> RVPPPPPCCHPRLSLHRPALEDLLLGSEANLTCTLTGLRDASGATFTWTPSSGKSAVQGPPERDLCGCYSVSSVLPGSAQPWNHGETFTCTAAHPELKTPLTATLSKSGNTFRPEVHLLPPPSEELALNELVTLTCLARGFSPKDVLVRWLQGSQELPREKYLTWASRQEPSQGTTTFFVYSILRVAAEDWKKGDTFSCMVGHEALPLAFTQKTIDRLAG;> RVPPPPPCCHPRLSLHRPALEDLLLGSEANLTCTLTGLRDASGATFTWTPSSGKSAVQGPPERDLCGCYSVSSVLPGSAQPWNHGETFTCTAAHPELKTPLTATLSKSGNTFRPEVHLLPPPSEELALNELVTLTCLARGFSPKDVLVRWLQGSQELPREKYVTTASRQEPSQGTTTFAVTSLLRVAAEDWKKGDTFSCMVGHEALPLAFTQKTIDRLAG;>KEKQERVQHLYDIKDLHRYYSSESFEFSNISGKVENYNGSNVVRFNQEKQNHQLFLLGEDKAKYKQGLQGQDVFVVKELIDPNGRLSTVGGVTKKNNQSSE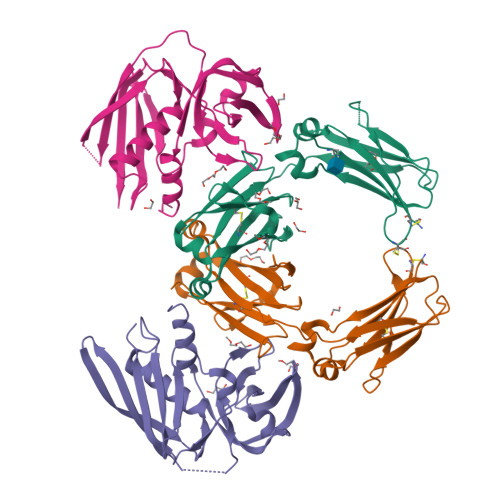TNIHLLVNKLDGGNLDATNDSFLINKEEVSLKELDFKIRKQLVEKYGLYQGTSKYGKITIILNGGKKQEIDLGDKLQFERMGDVLNSKDINKIEVTLKQI[2x]>[2x]SEFMKIAIAGAGAMGSRFGVKLQEAGNQVTLIDNWSAHVDQINQAGLTVTTDDGVDHVYTMTAQHPEAVTDQFDLIILFTKTMQMDAMLQQLAPVLTNHPIVLTLGNGIGNIETIERHVPKNQIVVGTTV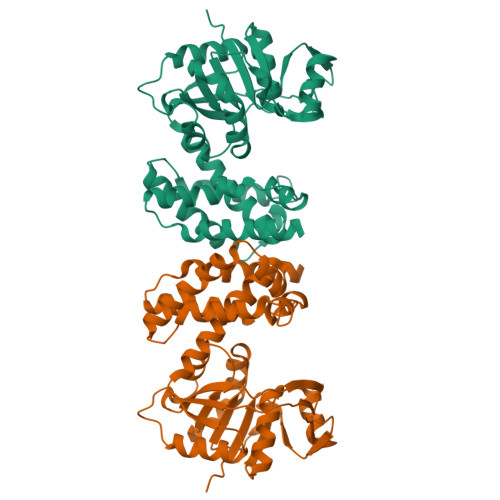WSSGLTGPGHITVTGGGSISLQAVVPDQFPNLADLITTLNAAGLNASAADNVLAAIWKKAGLNSVLNTYCTLFDCNIGEFGALKNWQTLTATVLDEFQAVADAAQIQFSAAAVTDLIAAQFPAAVNGNHYPSMHQDMANQRPTEIDFLNGYVAKLGQQLHVPTPANALLTQLIHSQEQLKQI> MLNQSKILTLQAYDPAKVLVFIGGQRVSGFA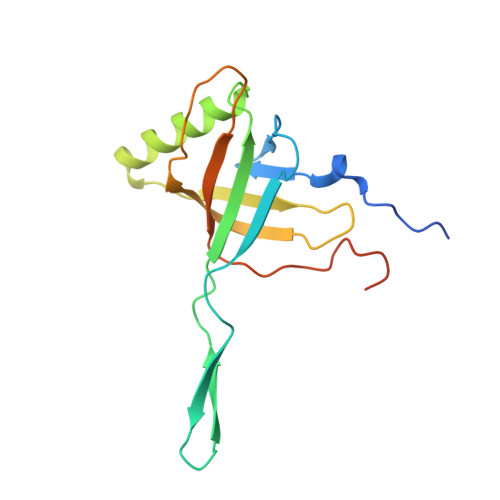ADTKIVITRNNDNISVHAGVDGEISNALSRDNTGVMTLSLQNTAKWNGYLAQWQRQANVTGLIYLPVQVEGSQGLSLNTIGWIQKQPDLSYGTEVGQMDWEIGVLDAWLSPDQIQGIAAGITGLLGLDQ> SQAEFDKAAEEVKHLKTKPADEEMLFIYSHYKQATVGDINTERPGMLDFKGKAKWDAWN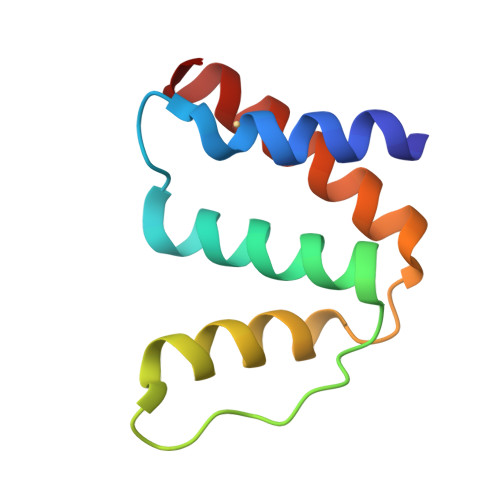ELKGTSKEDAMKAYIDKVEELKKKYGI> CLAEGTRIFDPVTGTTHRIEDVVDGR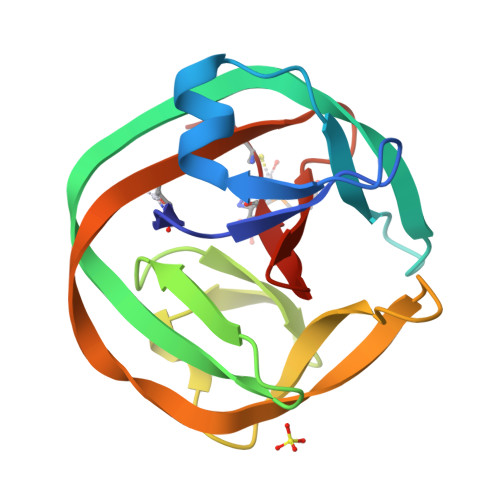KPIHVVAAAKDGTLHARPVVSWFDQGTRDVIGLRIAGGAILWATPDHKVLTEYGWRAAGELRKGDRVAVRDVETGELRYSVIREVLPTRRARTFDLEVEELHTLVAEGVVVHACSP>[5x]GSEKWTSTAIITQPDAAQVATYTNALNVLYGGNAPKISEVQANFISRFSSAFSALSEVLDNQKEREKLT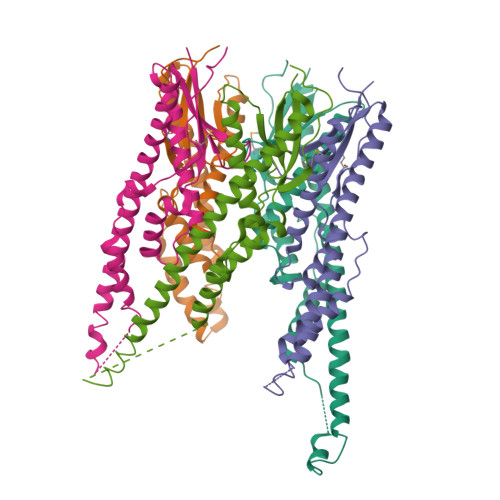IEQSVKGQALPLSVSYVSTTAEGAQRRLAEYIQQVDEEVAKELEVDLKDNITLQTKTLQESLETQEVVAQEQKDLRIKQIEEALRYADEAKITQPQIQQTQDVTQDTMFLLGSDALKSMIQNEATRPLVFSPAYYQTKQTLLDIKNLKVTADTVHVYRYVMKPTLPVRRDSPKT> MKKNGKSQNQPLDFTQYAKNMRKDLSNQDICLEDGALNHSYFLTKKGQYWTPLNQKALQRGIELFGVGNWKEINYDEFSGKANIVELELRTCMILGINDITE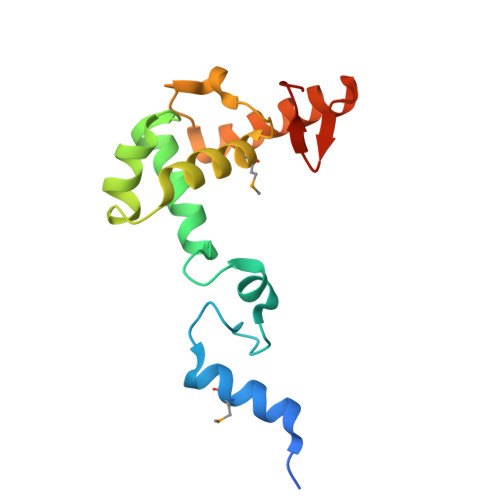YYGKKISEEEQEEIKKSNIAKGKKENKLKDNIYQKLQQMQ>[2x]MVKNWLFGKKRKEDADALATLKGQQNRLQAEARNLERQSDEQKILASKMLKAGNKAGARQALKRRAVFMKRLNTVHNTAMNLQAQIDSIQTATSTAETVKAMELGTKVVGEKIKTVSPERTERVMDSVMEQRDQIEMMTEALSDPSLSEGILDFEDDAAIDEQLAQLEAEMDLGTTTSLPDVSGLPSTPVGTGEKEEDTSELEAELEGLKKKMSEDKQ

To aid these processes, cells from across the tree of life use a conserved family of polymer-forming endosomal sorting complex required for transport III (ESCRT-III) proteins that deform, cut, and repair membranes (1–3). Individual ESCRT-III proteins are small and have a simple set of α helices (α1 to α5) that define the functional core of the protein. The most stripped-down version of the ESCRT-III system is found in Asgard archaea, the closest prokaryotic relatives of eukaryotes, which have as few as two ESCRT-III homologs. We show that Asgard ESCRT-IIIB assembles into parallel arrays on planar membranes to initiate membrane deformation, from where it recruits ESCRT-IIIA to generate composite polymers.

However, after mixing the protein with large unilamellar vesicles (LUVs) containing 40 mol % of the negatively charged lipid 1,2-dioleoyl-sn-glycero-3-phospho-l-serine (DOPS), long filaments were observed by cryo-EM. These filaments have a diameter of ~12 nm and are reminiscent of those formed by eukaryotic B-type ESCRT-III proteins. Filaments were also seen decorating and occasionally interacting with LUVs of various shapes, further suggesting that polymer nucleation is aided by the presence of membranes under these conditions. The polymers are composed of four protofilaments (blue, pink, green, and orange). (C) Top view of a cross section through the filament, highlighting the two protofilament pairs and the interprotofilament interactions through α1 and α4. A comparison with our off-membrane structure revealed a slightly smaller intersubunit distance in the membrane-bound protofilament (~3 nm versus 2.7 nm, respectively). This was accompanied by a change in the angle between helices α3 and α4 (off-membrane: 145°; on-membrane: 116°). Although the precise nature of Asgard cell membranes has yet to be determined, our data reveal a requirement for a critical concentration of ESCRT-IIIB protein to initiate polymer formation on reconstituted membranes. This likely reflects the need to form a stable five-subunit nucleus involving i to i + 4 interactions, which then extends by fast polymerization, as is the case for other cytoskeletal elements like actin.>[6x]MNYWIAATGALALAVAVTAQGTTLLHNAKAQVTTPCGASHYMRHITRQAESALQAGLKTAQSALETSNKLRVVASSKTGGAATAASILAANLASEAAKAIETIKTETKNFLAGFAAAAELAGQQTIVSEIKSAQVQDVNTLTAAQAVTTPGIIQVKPKLTIASTAACFNDDGSPVSDDEAAQPNQGEPTLKFFVVSANTPGTTHNELLTICGHGSTGTAPSTGCQNDATSIGIKGGDFLKTAAVTTTRLASSAGKTYPAITSTTTIPNDKTLNKAVTAIRELETAVAALDAISDVSSPEDIAARPELTEAIAKALDGDKAKVDSFAAETFGKESAIVKSTIVKDLKDLKPPKSAVGGSGEKKLETINDPKELADAQIYYTVKKFVDEQEQKKKNQASPSCPTNTDKTTEPAKSADECKKHTTSDDCKDEKGCEFDEKKDPKCFPKVDTEKKDDKSFSSNVRVSVPQVFAALVLAAF

Long-term immune evasion by the African trypanosome is achieved through repetitive cycles of surface protein replacement with antigenically distinct versions of the dense Variant Surface Glycoprotein (VSG) coat. The mature VSG proteins are attached to the cell surface by a GPI-anchor, and consist of two main regions: (1) a large, N-terminal domain (NTD) of roughly 300–400 amino acids that is most distal to the membrane and (2) a smaller, membrane-proximal C-terminal domain (CTD) spanning 80–120 amino acids beneath the NTD that harbors the GPI-anchor. Therefore, at the heart of antigenic variation in the African trypanosome are the NTDs of the VSGs. These large subdomains are elongated folds centered on a three-helix bundle scaffold.

The structures of VSG21 and VSG545 were also determined, both harboring closely related folds and biochemical properties that distinguish them from other VSGs. Of note is the fact that both structures were obtained with proteolytic removal of the bottom lobe (contained in the C-terminal region of the NTD sequence). This cleavage occurred spontaneously during crystallization experiments performed with full-length VSG21 and the NTD of VSG545 that had been produced by limited proteolysis with Endoproteinase Lys-C (LysC). In contrast, for VSG21 and VSG545, the cleavage in the crystallization drops produced a truncated NTD missing the bottom lobe sequence but maintaining the 3-helix bundle and top lobe of the protein. No sugar is seen in the VSG21 electron density, and no predicted site for N-linked glycosylation (Asn-Xaa-Ser/Thr) was found in the sequence of the NTD. VSG21 and VSG545 are more similar to each other than these other VSGs, however, distinguished from them by the tightly twisted nature of the top lobe and, directly beneath it, the presence of a second three-stranded beta-sheet perpendicular to the axis of the 3-helix bundle. VSG21 and VSG545 align well to each other in the top lobe but not to the other VSGs with beta-sheet top lobes. Superpositions with predicted models from AlphaFold (which were accurate enough to solve the experimental structures by molecular replacement) show possible conformations of the full NTD for each protein. In this subdivision, we split the A3 class from Cross into A1b and A1c (which correspond to classes N5 and N3 in Weirather, respectively) based on differences in the top lobe architecture (e.g., the smaller top lobe beta-sandwich in A1c compared to A1b and the presence of a second beta-sheet over the middle lobe in A1c that is not present in A1b).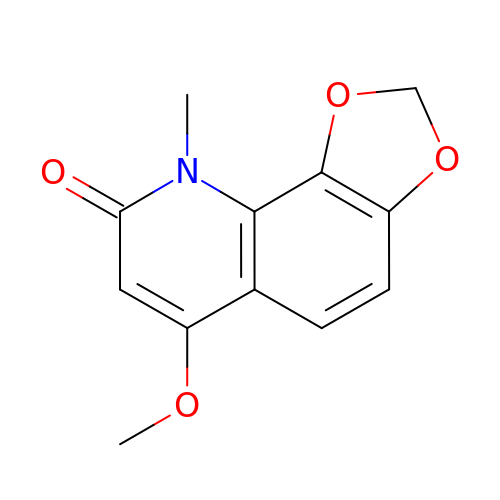6-methoxy-9-methyl[1,3]dioxolo[4,5-h]quinolin-8(9H)-one | C12 H11 N O4 | DPXXJCMMMXZVSW-UHFFFAOYSA-N> GHIKQLLKNKRFEVIKALVESKKIKQEWLEDLYSILLKQDTDVEITQAKYEIIKLLLTEKKYLNFELLTKTLNLDQQTAIEIMRNPFKEVYFPTYNIENPEESRLNKALIIPLSNQTFTLNTFVNSQDLETIKEATNKNFFVIFDNIFSGKSYQLAVAAGLIAKEKEILDNVAFTGEVSSNGFIIPVNHLEEKKEITEKAKKVLITPEDIENLEELSFWLNPEHLPVIFIHINKPELALQSL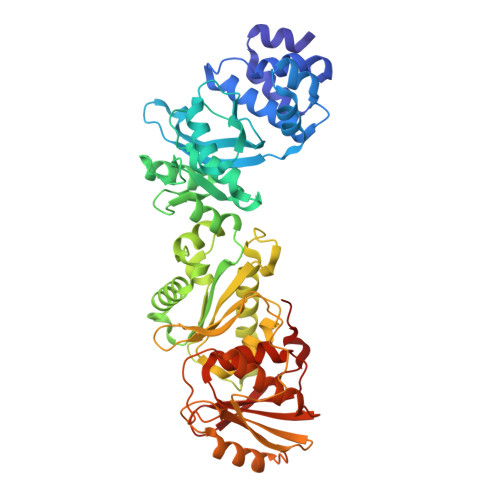KQMEDAIKKDERFKYFKLENLKKFYRLEDQDMYLITPSVDFSNREELIKILNEFREKVSKLLTLEGVIKDHNKVVLNISAGISTLALYFGVILGNRQASIIYHYQKEYHKVIDLTDNPRKIKEKKSEFEKISVNKNIQDPLMIIIYLASHNPIEKGLELKEKLRAKGELIIQSKEHQGNLEIGDWSDIVSEIYTAIDDNKQKENYMVFSAPVAIMLALGMALGYFLPIKVFHYNRDEYIEVPIKLNEEILRSPF> RGLASKKTTTVGVIIPDISNIFYAELARGIEDIATMYKYNIILSNSDQNQDKELHLLNNMLGK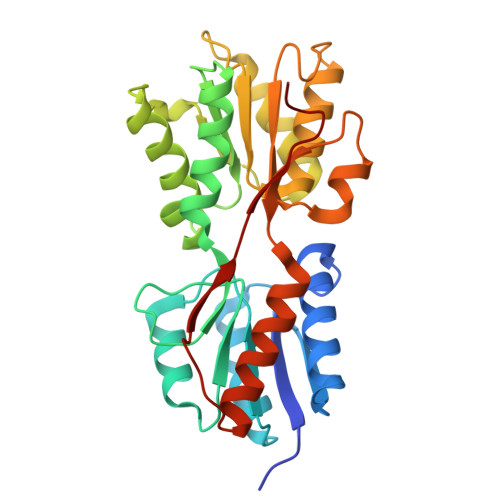QVDGIIFMSGNVTEEHVEELKKSPVPVVLAASIESTNQIPSVTIDYEQAAFDAVQSLIDSGHKNIAFVSGTLEEPINHAKKVKGYKRALTESGLPVRDSYIVEGDYTYDSGIEAVEKLLEEDEKPTAIFVGTDEMALGVIHGAQDRGLNVPNDLEIIGFDNTRLSTMVRPQLTSVVQPMYDIGAVAMRLLTKYMNKETVDSSIVQLPHRIEFRQSTK The Arabidopsis VEL proteins are accessory proteins that interact with PRC2 to nucleate and propagate silencing at the FLOWERING LOCUS C (FLC) locus, enabling early flowering in spring. Here, we report that VEL proteins contain a domain related to an atypical four-helix bundle that engages in spontaneous concentration-dependent head-to-tail polymerization to assemble dynamic biomolecular condensates. The VEL domain adopts a compact globular fold, consisting of four α-helices in a quasi-antiparallel “up-down-up-down” configuration, each of which contributes to the hydrophobic core, as illustrated by VEL1VEL. Mutations blocking polymerization of this VEL domain prevent Polycomb silencing at FLC.

The equivalent double mutation of VEL1VEL (RK>AD) also essentially blocks polymerization. In a subsequent round of mutation screening based on crystal structures (see below), we identified four additional substitutions of conserved surface-exposed residues of VIN3VEL that strongly attenuated (R541H, R556D, L563D) or blocked (I575D) polymerization. As expected, the head mutations L563D, R541H, and T559E and the tail mutation I575D all reduce or abolish self-association without affecting the protein expression levels. As expected, these interacting residues are all invariant or semi-conserved, except for I575, whose counterparts are also hydrophobic in VIN3 paralogs but are typically threonines in VRN5 paralogs. VIN3VEL crystals also show protofilaments; however, these are invariably composed of dimers rather than monomers as in VEL1VEL. Indeed, dimers are seen in every single crystal, regardless of the mutant, space groups, or crystallization conditions. Interestingly, these dimers result from mutual domain swapping of H4 between individual VIN3VEL monomers whereby molecule A donates its H4 to molecule B in an adjacent VIN3VEL filament, and vice versa. To form filaments, individual VIN3VEL dimers either stack perpendicularly on top of each other in a “cruciform” fashion (in RR>AD) or they associate pairwise to form tetramers that, in turn, stack pairwise along the polymerization axis (in I575D).

>[4x]GDKDLGHIVKTIRCLEEEGHIDKSFRERFLTWYSLRATHREVRVVKDFVETFMEDLSSLGQQLVDTFSESILSKR>VTAFLGERVTLTSYWRRVSLGPEIEVSWFKLGPGEEQVLIGRMHHDVIFIEWPFRGFFDIHRSANTFFLVVTAANISHDGNYLCRMKLGETEVTKQEHLSVVKPLTLSVHSERSQ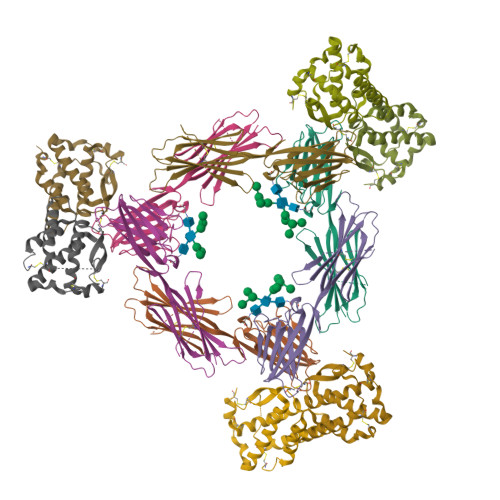FPDFSVLTVTCTVNAFPHPHVQWLMPEGVEPAPSAANGGVMKEKDGSLSVAVDLSLPKPWHLPVTCVGKNDKEEAHGVYVSGYLSQKHHHHHH[12x];>GSHMEEVSEYCSHMIGSGHLQSLQRLIDSQMETSCQITFEFVDQEQLKDPVCYLKKAFLLVQDIMEDTMRFRDNTPNAIAIVQLQELSLRLKSCFTKDYEEHDKACVRTFYETPLQLLEKVKNVFNETKNLLDKDWNIFSKNCNNSFAECSSQ[12x]>[2x]MSKTQEFRPLTLPPKLSLSDFNEFIQDIIRIVGSENVEVISSKDQIVDGSYMKPTHTHDPTHVMDQDYFLASAIVAPRNVADVQSIVGLANKFSFPLWPISIGRNSGYGGAAPRVSGSVVLDMGKNMNRVLEVNVEGAYCVVEPGVTYHDLHNYLEANNLRDKLWLDVPDLGGGSVLGNAVERGVGYTPYGDHWMMHSGMEVVLANGELLRTGMGALPDPKRPETMGLKPEDQPWSKIAHLFPYGFGPYIDGLFSQSNMGIVTKIGIWLMPNPGGYQSYLITLPKDGDLKQAVDIIRPLRLGMALQNVPTIRHILLDAAVLGDKRSYSSRTEPLSDEELDKIAKQLNLGRWNFYGALYGPEPIRRVLWETIKDAFSAIPGVKFYFPEDTPENSVLRVRDKTMQGIPTYDELKWIDWLPNGAHLFFSPIAKVSGEDAMMQYAVTKKRCQEAGLDFIGTFTVGMREMHHIVCIVFNKKDLIQKRKVQW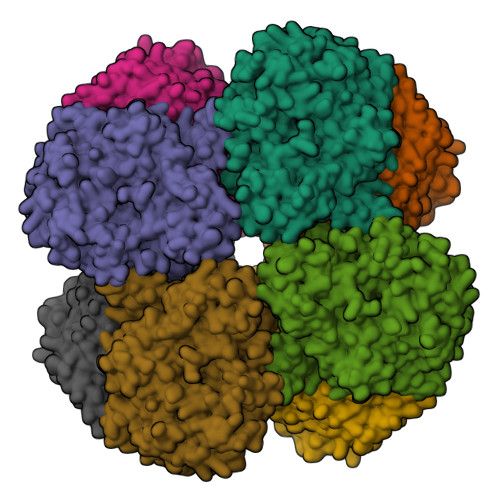LMRTLIDDCAANGWGEYRTHLAFMDQIMETYNWNNSSFLRFNEVLKNAVDPNGIIAPGKSGVWPSQYSHVTWKL>GSVYMLFIDIEVNGVPIKAFVDSGAQSTFMSYACAQKCSLLRLMDTRYRGVAQGVGKTEIVGKIHLATLKIGQRFFPSSFTVLQDNKVEF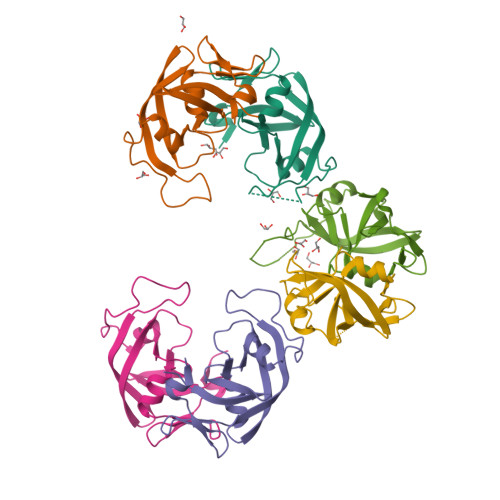LFGLDLLRRYQCCIDLKKSVLRIDNEEIPFLSEKDITK[12x]> GGPGPRVLVVGSGIAGLGAAQKLCSHRAAPHLRVLEATASAGGRIRSERCFGGVVELGAHWIHGPSQDNPVFQLAAEFGLLGEKELSEENQLVDTGGHVALPSMIWSSSGTSVSLELMTEMARLFYGLIERTREFLNESETPMASVGEFLKKEISQQVASWTEDDEDTRKRKLAILNTFFNIECCVSGTHSMDLVALAPFGEYTVLPGLDCILAGGYQGLTDRILASLPKDTVAFDKPVKTIHWNGSFQEAAFPGETFPVLVECEDGARLPAHHVIVTVPLGFLKEHQDTFFEPPLPAKKAEAIKKLGFGTNNKIFLEFEEPFWEP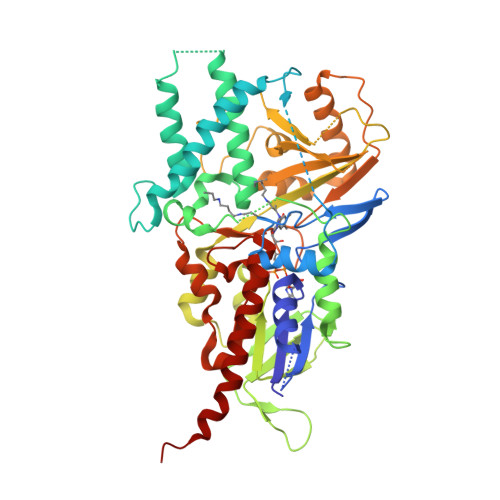DCQFIQVVWEDTSPLQDTALSLQDTWFKKLIGFLVQPSFESSHVLCGFIAGLESEFMETLSDEEVLLSLTQVLRRVTGNPQLPAAKSVRRSQWHSAPYTRGSYSYVAVGSTGDDLDLMAQPLPGLQVLFAGEATHRTFYSTTHGALLSGWREADRLVSLWDSQVEQSRPRL>MGSSHHHHHHSSGLVPRGSHGFEFNIMVVGQSGLGKSTLINTLFKSKISRKSVQPTSEERIPKTIEIKSITHDIEEKGVRMKLTVIDTPGFGDHINNENCWQPIMKFINDQYEKYLQEEVNINRKKRIPDTRVHCCLYFIPATGHSLRPLDIEFMKRLSKVVNIVPVIAKADTLTLEERVHFKQRITADLLSNGIDVYPQKEFDEDSEDRLVNEKFREMIPFAVVGSDHEYQVNGKRILGRKTKWGTIEVENTTHCEFAY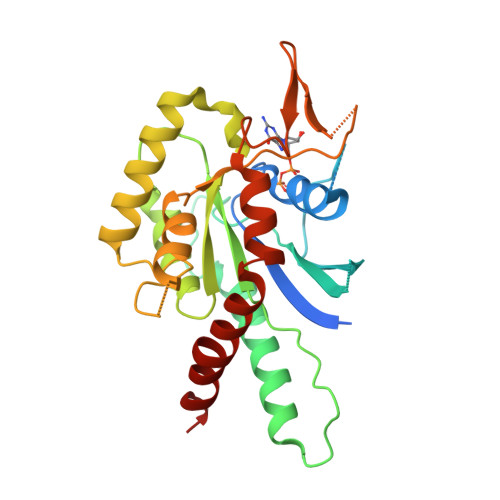LRDLLIRTHMQNIKDITSSIHFEAYRVKRL[2x]> MMYIQVLGSAAGGGFPQWNCNCVNCKGYRDGTLKATARTQSSIALSDDGVHWILCNASPDIRAQLQAFAPMQPARALRDTGINAIVLLDSQIDHTTGL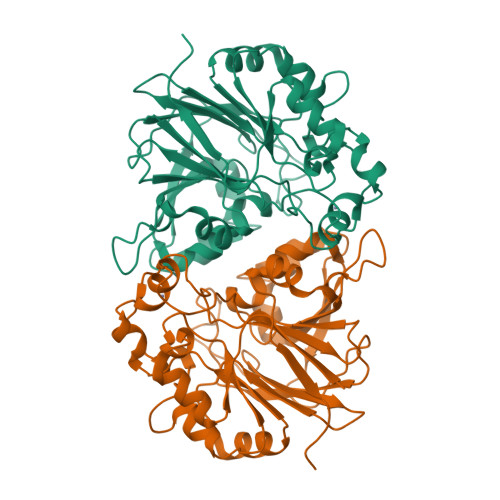LSLREGCPHQVWCTDMVHQDLTTGFPLFNMLSHWNGGLQWNRIELEGSFVIDACPNLKFTPFPLRSAAPPYSPHRFDPHPGDNLGLMVEDTRTGGKLFYAPGLGQVDEKLLAMMHGADCLLVDGTLWEDDEMQRRGVGTRTGREMGHLAQNGPGGTLEVLDGFPRQRKVLIHINNTNPILDENSPERAEVLRRGVEVAFDGMSIELLEHHH>[4x]ADPGGSHHHHHHSRKTYTLTDYLKNTYRLKLYSLRWISDHEYLYKQENNILVFNAEYGNSSVFLENSTFDEFGHSINDYSISPDGQFILLEYNYVKQWRHSYTASY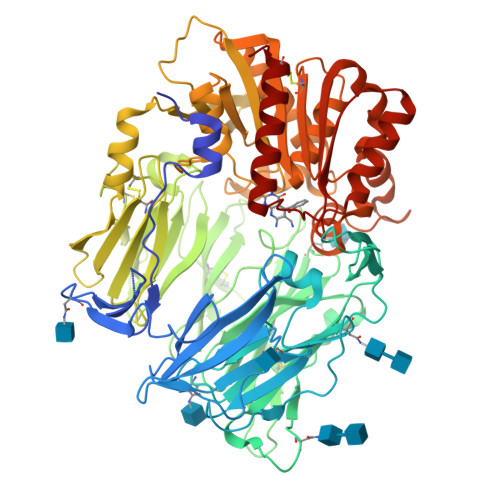DIYDLNKRQLITEERIPNNTQWVTWSPVGHKLAYVWNNDIYVKIEPNLPSYRITWTGKEDIIYNGITDWVYEEEVFSAYSALWWSPNGTFLAYAQFNDTEVPLIEYSFYSDESLQYPKTVRVPYPKAGAVNPTVKFFVVNTDSLSSVTNATSIQITAPASMLIGDHYLCDVTWATQERISLQWLRRIQNYSVMDICDYDESSGRWNCLVARQHIEMSTTGWVGRFRPSEPHFTLDGNSFYKIISNEEGYRHICYFQIDKKDCTFITKGTWEVIGIEALTSDYLYYISNEYKGMPGGRNLYKIQLSDYTKVTCLSCELNPERCQYYSVSFSKEAKYYQLRCSGPGLPLYTLHSSVNDKGLRVLEDNSALDKMLQNVQMPSKKLDFIILNETKFWYQMILPPHFDKSKKYPLLLDVYAGPCSQKADTVFRLNWATYLASTENIIVASFDGRGSGYQGDKIMHAINRRLGTFEVEDQIEAARQFSKMGFVDNKRIAIWGWSYGGYVTSMVLGSGSGVFKCGIAVAPVSRWEYYDSVYTERYMGLPTPEDNLDHYRNSTVMSRAENFKQVEYLLIHGTADDNVHFQQSAQISKALVDVGVDFQAMWYTDEDHGIASSTAHQHIYTHMSHFIKQCFSLP>[26x]FTLIELMIVIAIVGILA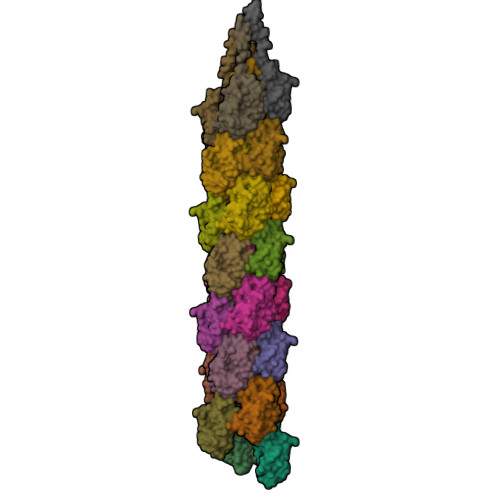AVALPAYQDYTARAQVSEAILLAEGQKSAVTEYYLNHGEWPGDNSSAGVATSADIKGKYVQSVTVANGVITAQMASSNVNNEIKSKKLSLWAKRQNGSVKWFCGQPVTRTTATATDVAAANGKTDDKINTKHLPSTCRDDSSAS>SPGVVISDDEPGYDLDLFCIPNHYAEDLERVFIPHGLIMDRTERLARDVMKEMGGHHIVALCVLAGGYKFFADLLDYIKALNRNSDRSIPMTVDFIRLGSYCNDQSTGDIKVIGGDDLSTLTGKNVLIVEDIIDTGKTMQTLLSLVRQY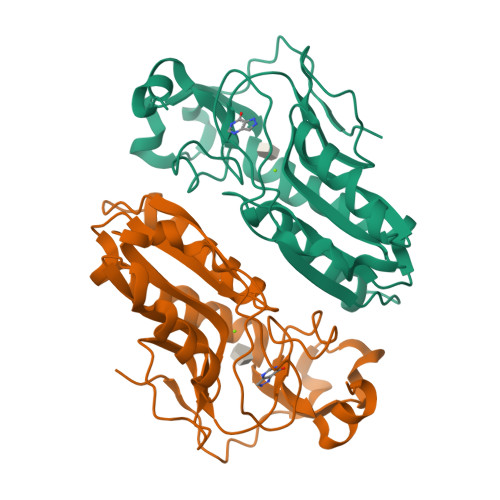NPKMVKVASLLVKRTPRSVGYKPDFVGFEIPDKFVVGYALDYNEYFRDLNHVCVISETGKAKYKA[2x]> GCSDGSGWSS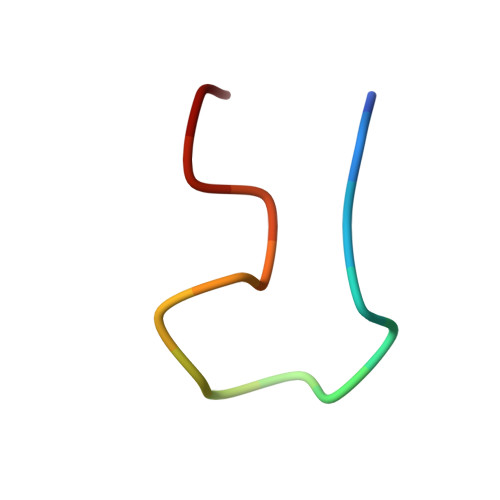ENNPWG>[2x]MAHHHHHHSAALEVLFQGPGMASGSNVEEYELDVEALVVILRDRNIPRNPLHGEVIGLRLTEGWWGQIERFQMVRLILQNDDNEPLQRPRYEVIQRAVNPHTMFMISGPLAELQLAFQDLDLPEGPLRFGPLANGHYVQGDPYSSSYRPVTMAETAQMTRDELEDVLNTQSEIEIQMINLLELYEVETRALRRQLAERS

PFV Gag is a 648 polypeptide and the major FV structural protein in the assembled virion. Moreover, in all retroviral subfamilies Gag carries out the same functional roles including assembly, nucleic acid packaging, transport to and budding through the cytoplasmic membrane of the producer cell as well as trafficking through the cytoplasm of the target cell and uncoating. Here we report the crystal structure an amino terminal domain from the Gag of PFV (PFV-Gag-NtD), provide the molecular details of the interaction of this domain with the N-terminal leader sequence from the PFV Envelope (PFV-Env) and demonstrate that the PFV-Gag-NtD is also the target for Trim5α restriction factors. Our data reveal that the FV Gag is unique and structurally unrelated to the Gag protein of other retroviruses.

Bioinformatic analysis of the primary sequence and that of related FVs suggested that the N-terminal 179 residues of PFV-Gag comprised a stable domain (PFV-Gag-NtD). This fragment was expressed in E. coli and subsequently the crystal structure determined by SAD methods and refined at a resolution of 2.4 Å. The final Rwork/Rfree are 17.2% and 23.0% respectively. By comparison, our data reveals the PFV-Gag-NtD to be entirely unrelated comprising a mixed α/β protein with head and stalk domains. The PFV-Gag-NtD dimer interface buries approximately 1700 Å2 of the monomer surface area. The large central coiled-coil formed by helix α6 comprises the majority of this interface, supplemented by residues in helices α4 and α5 and the adjoining loop. The coiled-coil contains three regions of leucine zipper at residues Leu143/147, Leu160/161 and Leu171/175. Additionally, a highly synergistic hydrogen-bonding network centred on residue Glu154 is located between two of the zipper regions. Here, the Glu154 sidechain forms hydrogen bonds with the sidechains of Glu154*, Gln150* and Tyr127* of the opposing monomer. In FVs the proposed CTRS constitutes residues 43 to 60 of the PFV-Gag-NtD where residues Leu40 to Arg50 form the loop that links β1 to β2 and the remainder make up the β2 strand.>[2x]AKIDNAVLPEGSLVLVTGANGFVASHVVEQL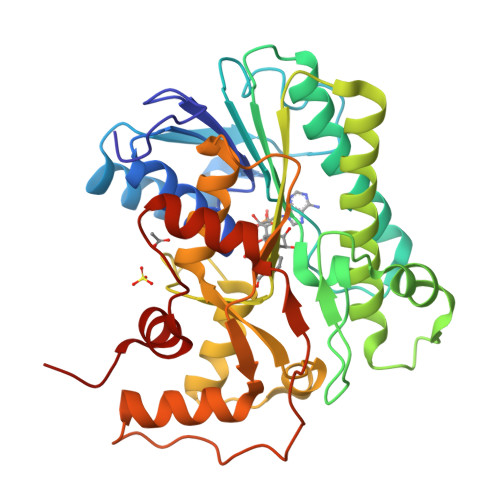LEHGYKVRGTARSASKLANLQKRWDAKYPGRFETAVVEDMLKQGAYDEVIKGAAGVAHIASVVSFSNKYDEVVTPAIGGTLNALRAAAATPSVKRFVLTSSTVSALIPKPNVEGIYLDEKSWNLESIDKAKTLPESDPQKSLWVYAASKTEAELAAWKFMDENKPHFTLNAVLPNYTIGTIFDPETQSGSTSGWMMSLFNGEVSPALALMPPQYYVSAVDIGLLHLGCLVLPQIERRRVYGTAGTFDWNTVLATFRKLYPSKTFPADFPDQGQDLSKFDTAPSLEILKSLGRPGWRSIEESIKDLVGSETA>[2x]GPGGHMANFDFDVWRKKYMRWMNHKKSRVMDFFRRIDKDQDGKITRQEFIDGILASKFPTTKLEMTAVADIFDRDGDGYIDYYEFVAALHP;> DADKIEDEVTRQVAQCK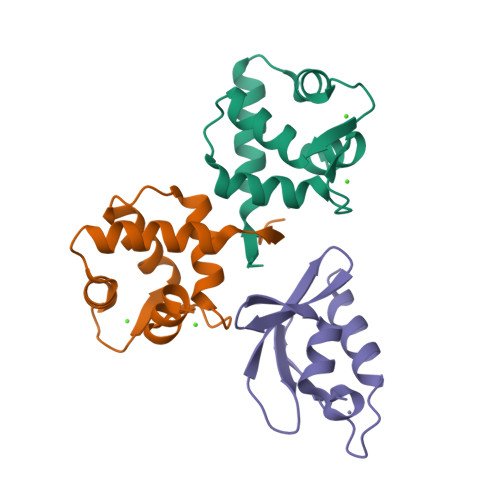CAKRFQVEQIGENKYRFGDSQQLRLVRILRSTVMVRVGGGWMALDEFLVKNDPCRAR> NCSKIHLSTKLLAVDFPAHFVKSISCQICEHILADPVETSCKHLFCRICILRCLKVMGSYCPSCRYPCFPTDLESPVKSFLNILNSLMVKCPAQDCNEEVSLEKYNHHVSSHKESKETLVHINKGGRPRQHLLSLTRRAQKHRLRELKIQVKEFADKEEGGDVKAVCLTLFLLALRARNEHRQADELEAIMQGRGSGLQPAVCLAIRVNTFLSCSQYHKMYRTVKAITGRQIFQPLHALRNAEKVLLPGYHPFEWQPPLKNVSSRTDVGIIDGLSGLASSVDEYPVDTIAKRFRYD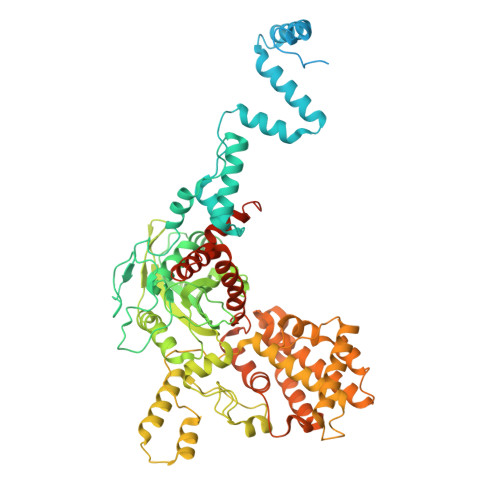SALVSALMDMEEDILEGMRSQDLDDYLNGPFTVVVKESCDGMGDVSEKHGSGPAVPEKAVRFSFTVMRITIEHGSQNVKVFEEPKPNSELCCKPLCLMLADESDHETLTAILSPLIAEREAMKSSELTLEMGGIPRTFKFIFRGTGYDEKLVREVEGLEASGSVYICTLCDTTRLEASQNLVFHSITRSHAENLQRYEVWRSNPYHESVEELRDRVKGVSAKPFIETVPSIDALHCDIGNAAEFYKIFQLEIGEVYKHPNASKEERKRWQATLDKHLRKRMNLKPIMRMNGNFARKLMTQETVDAVCELIPSEERHEALRELMDLYLKMKPVWRSSCPAKECPESLCQYSFNSQRFAELLSTKFKYRYEGKITNYFHKTLAHVPEIIERDGSIGAWASEGNQSGNKLFRRFRKMNARQSKCYEMEDVLKHHWLYTSKYLQKFMNAHNALKSSGFTMNSKETLGDPLGIEDSLESQDSME> MPVRRGHVAPQNTFLDTIIRKFEGQSRKFIIANARVENCAVIYCNDGFCELCGYSRAEVMQRPCTCDFLHGPRTQRRAAAQIAQALLGAEERKVEIAFYRKDGSCFLCLVDVVPVKNEDGAVIMFILNFEVVMEKDMVGSSPTSDREIIAPKIKERTHNVTEKVTQVLSLGADVLPEYKLQAPRIHRWTILHYSPFKAVWDWLILLLVIYTAVFTPYSAAFLLKETEEGPPATECGYACQPLAVVDLIVDIMFIVDILINFRTTYVNANEEVVSHPGRIAVHYFKGWFLIDMVAAIPFDLLIFGSGSEELIGLLKTARLLRLVRVARKLDRYSEYGAAVLFLLMCTFALIAHWLACIWYAIGNMEQPHMDSRIGWLHNLGDQIGKPYNSSGLGGPSIKDKYVTALYFTFSSLTSVGFGNVSPNTNSEKIFSICVMLIGSLMYASIFGNVSAIIQRLYSGTARYHTQMLRVREFIRFHQIPNPLRQRLEEYFQHAWSYTNGIDMNAVLKGFPECLQADICLHLNRSLLQHCKPFRGATKGCLRALAMKFKTTHAPPGDTLVHAGDLLTALYFISRGSIEILRGDVVVAILGKNDIFGEPLNLYARPGKSNGDVRALTYCDLHKIHRDDLLEVLDMYPEFSDHFWSSLEITFNLRDTNMIPGGRQYQELPRCPAPTPSLLNIPLSSPGRRPRGDVESRLDALQRQLNRLETRLSADMATVLQLLQRQMTLVPPAYSAVTTP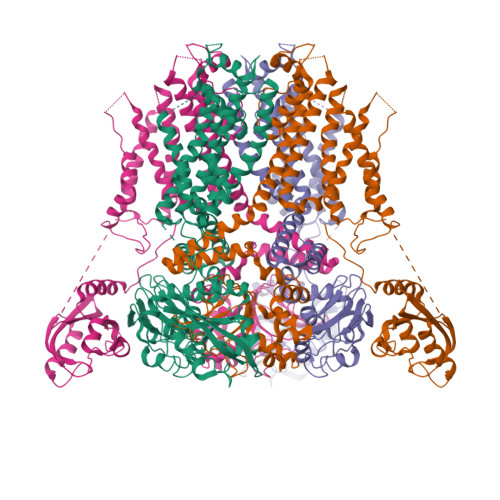GPGPTSTSPLLPVSPLPTLTLDSLSQVSQFMACEELPPGAPELPQEGPTRRLSLPGQLGALTSQPLHRHGSDPGSEASNSLEVLFQ> SNAQVQVGAPEEEEEEEEDAGLVAEAEAVAAGWMLDFLCLSLCRAFRDGRSEDFRRTRNSAEAIIHGLSSLTACQLRTIYICQFLTRIAAGKTLDAQFENDERITPLESALMIWGSIEKEHDKLHEEIQNLIKIQAIAVCMENGNFKEAEEVFERIFGDPNSHMPFKSKLLMIISQKDTFHSFFQHFSYNHMMEKIKSYVNYVLSEK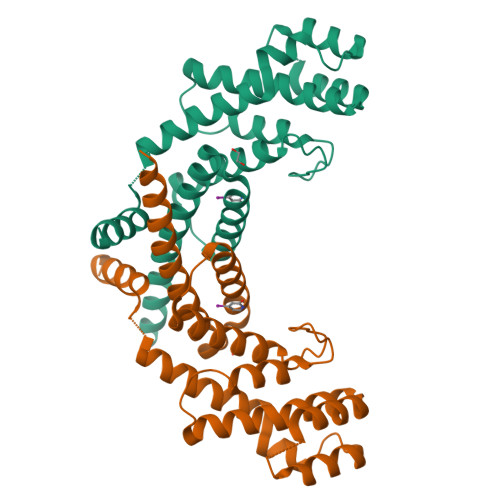SSTFLMKAAAKVVESKR[(1S)-4-[hydroxy(methyl)amino]-1-(4-methoxyphenyl)-4-oxobutyl]phosphonic 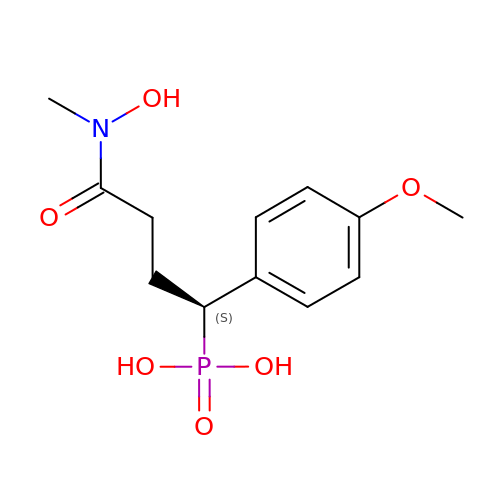acid | C12 H18 N O6 P | VLBYPFQOJHBTHH-NSHDSACASA-N Clostridium histolyticum collagenases ColG and ColH are segmental enzymes that are thought to be activated by Ca2+-triggered domain reorientation to cause extensive tissue destruction. The collagenases consist of a collagenase module (s1), a variable number of polycystic kidney disease-like (PKD-like) domains (s2a and s2b in ColH and s2 in ColG) and a variable number of collagen-binding domains (s3 in ColH and s3a and s3b in ColG). The X-ray crystal structures of Ca2+-bound holo s2a (space group C2), Ca2+-free apo s2a (space group P61), Ca2+-bound holo s2b (space group P21) and two new forms of N-terminally truncated wild-type apo s2 (space groups P21 and P212121) are reported for the first time. Comparison of crystal structures of ColG s2 with crystal structures of ColH s2a and s2b suggests that despite common tertiary folds, PKD-like domains can be grouped into two subsets.

Despite being solved in two crystal forms, the crystal structures of forms I and II of apo s2 from ColG are similar. Each asymmetric unit contains two noncrystallographic twofold symmetry-related molecules. All four molecules are virtually identical to each other (r.m.s.d. of <0.5 Å). Each structure begins at residue 685, although the first two residues (Gly-Ser) are remnants from GST-tag cleavage. The last residue is either 770 or 771. In apo s2, intermolecular antiparallel β-sheet interactions involving β-strand A could suppress dynamics of the region. Conversely, the PKD-like domain of collagenases consisting of multiple CBDs, such as s2, appears to have no surface aromatic residues. In contrast, the subset containing s2 is likely to be different; the lack of surface aromatic residues on s2 suggests that the domain is less directly involved in interactions with collagen. In this context, the spring-like dynamics of s2 may allow it to swell the fibril.

>GSAPIAKVTGPSTGAVGRNIEFSGKDSKDEDGKIVSYDWDFGDGATSRGKNSVHAYKKAGTYNVTLKVTDDKGATATESFTIEIKNE[2x]NETROPSIN | C18 H26 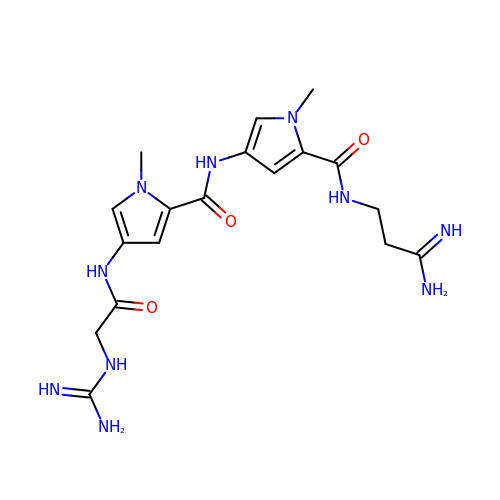N10 O3 | IDBIFFKSXLYUOT-UHFFFAOYSA-N> MSSAFSGLKIPELSVDPAEVFKSDNPQLVSVLLDEFELQEQRPFFSGLIPEKQINIALKKSPQLKKLACHLLEAYEINGRRWKHADRRRVLEKAIRLLEKVSNELKGDIQKLENNVKESGKDSEELNKTREKHGEILADMGRAYLHRAKII;> MGSSHHHHHHSQDPMQHIIPLTITFLESFRVIEWHKSSDRNSLRFLRGYAYARWHRSLKNNKGRPYITGTLVRSAIIRAAEELLWLNDGNYKGAICCPGEFNGSNAKVFREGKARRLRRRQTLTWPTKCACHEKEPCPFCLLLGRYEKSSKTSKSPVLNNVNFSNFNVLGKEKEFLNIEDVADMRVVNRVDQQSGKAEDFFNIWEITDGAWKIFRGEIQVSDKGWSDEENFSKFLTLLKGASVLVDKISGGLCYLTLDKPELAELPAVKTEKDVLEPGDDASVLEISRPPYWNNMLNLAGTISEAFEREDKLVHLRLFADTVRELRRSDIETLDLPKGHADRLGKPSDHFIWDIEINKKVKLRNWLFWIFNEFRDTYAYFDWRTFCEALGQALYLEAKKQVPNQFSSERPVGATPAMEVKTPEHDPGRAAQGPRYEWLIKGELVSQTPFFFGWSTEADNREHTNLKLLAARDGRLRLPLSVLR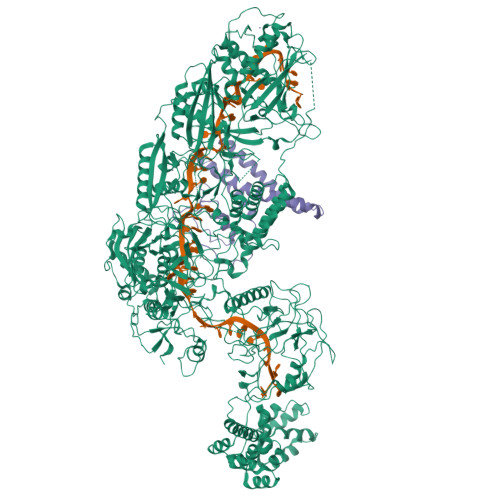GILRRDIKVVLDNKCRAELAMKQPCSCPVCNLMKKITIRDSFSSNYAEPPKIRHKIRLDPKSGTVAKGALFDSEVGPRGVVFPFELRLRSADDTLPQALKTVFSWWQQGTVSFSGDAGTGKGIFCLRNLKSIRWDLKTEMDKYAATLGGRKTPVGKWDKCHIPDDKTYPWVKETVEISVCSPFITKDPVNSLIDSAGYDAICYTTVDLEKSENINSLPESEISLLFEMFDLQYPMSYLFPNKDIYLLKGESFRGMLRTAVGRGENLLLREHEDCSCTLCRIFGNEHNAGKIRVEDFIIQGEPRTKLVDRVAIDRFTAGAKDKFKFDAAPIVGTPTNKLKFRGNIWIHRDLDGLACESLKLALEDIENGLYPFGGLGNAGFGWVNYNPLSHPAQEENKADFSLTKKMELNWSMKELSTDKIYWPHYFLPFGKKVLREKTPPSHACIDENEDSELYSGKIVCTLETRTPLIIPDSEFQGEEHKSYDFFNLNGELCIPGSEIRGMISSVFEALTNSCMRIFDEKKRLSWRMNPNKKDKKNNNRRELDDFIPGRVTNDRKMEEMKEYRYPFYDQAITANDKQNKYFDQWEATIELTDESLEKLKAEKILQSVLDALRPLTKKKEKYKNTETFVFDLKKFIGKIDDNQQMISEALERGKVRLTGNSLKQISKTKKIPRQILNQLKGLKDNTYENREQFISVLKTTVRGINDEQISLILDNIDEDVRLTDLSLTKIRKAKVPQTLVDMLADLKKDEPYKNEKEFLSEFKKKMGEIIGLILKHAAKTGGDVPRYNHPTPTDKMLLSLAAYNRNHKHENGKAEYRIVKPKHNLKVDFMFAVTPFENPFKGYNPAAVVEEPVGGYLKVSGPNKIEKVKKVNPNSVSVRDDKNQEIIHNGVYLRKITVANAKSKNKLRERLVPEFAWYDKDSEAAYAMTKRCERVFVEIGAKPIPIQPSAREKFKILTQEYQKNAKQQKTPEAFQTILPKDGELRPGDLVYFREDKKTNTVTDIIPVRISRTVDDEVLARKIPDDVGDVRPCVREILDKEKQKEIADAGVKEVFQHHPDGLCPACSLFGTTFYKGRIAFGFAFHKDKDPELANNGKHITLPLLERPRPTWSMPKKESRVPGRKFYVHHQGWERVIKHSNLDESDPNATKQTVNNRSVQAIKEEQKFQFEVRFENLREWELGLLVYVLQLEPQFAHKLGMGKALGFGSVRIRVGEIHSGPKELDESRLVSSAMKKMEEIWDRDKNVLEKLFRLLYFNESKDIKVRYPKLQKEKEEEEEESGYMELAKEEYQPEQRRNKLTNPWEGWGNILKKPAILI N-[(1S,2R)-2-hydroxy-1-(hydroxycarbamoyl)propyl]-4-(4-phenylbuta-1,3-diyn-1-yl)benzamide 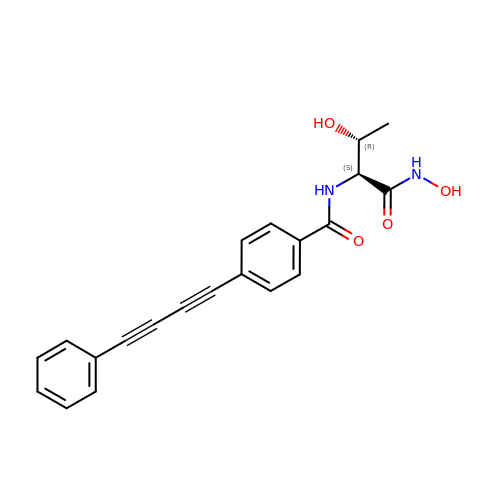| C21 H18 N2 O4 | VUYMSCCEGRLBAF-BEFAXECRSA-N> GCCCGGAUAGCUCAGUCGGUAGAGCAUCAGACUUUUAAUCUGAGGGUCCAGGGUUCAAGUCCCUGUUCGGGC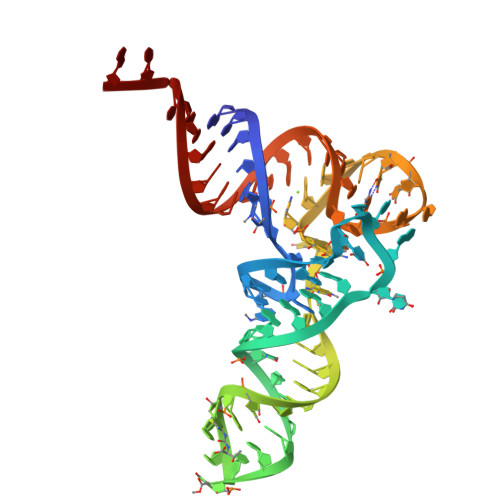GCCA>GSHMKPGFLYTIGLSNKGMPGLYRLELQVTKGSGKLATSGLWNSSSAKEQVKIAFDYFKANASRISGGSKVMEHDFHLHVVELQNTGPLSHLALPSLVAFASGLLGRSVQSQMVVLGDMSLGGSVTPVESIA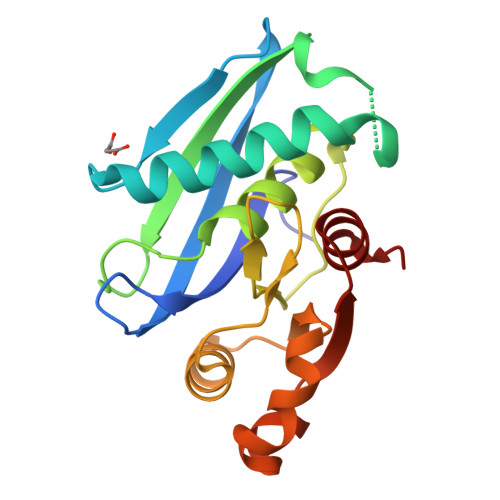ECLQVAFDAGAKKVALPMSSAADIPTIPVELFTKFQTSFYADPVDAVFKGLGVD[4x]>MGSSHHHHHHSQDPLVPRGSWETEERPRTREEECHFYAGGQVYPGEASRVSVADHSLHLSKAKISKPAPYWEGTAVIDGEFKELKLTDYRGKYLVFFFYPLDFTFVCPTEIIAFGDRLEEFRSINTEVVACSVDSQFTHLAWINTPRRQGGLGPIRIPLLSDLTHQISKDYGVYLEDSGHTLRGLFIIDDKGILRQITLNDLPVGRSV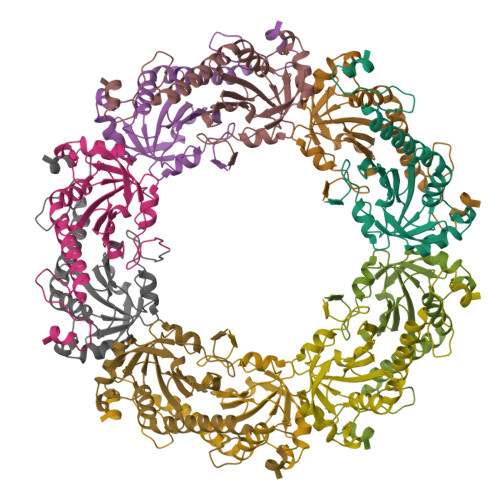DETLRLVQAFQYTDKHGEVAPAGWKPGSETIIPDPAGKLKYFDKLN[5x]> MSRSQLTILTNICLIEDLETQRVVMQYRAPENNRWSGYAFPGGHVENDEAFAESVIREIYEETGLTIQNPQLVGIKNWPL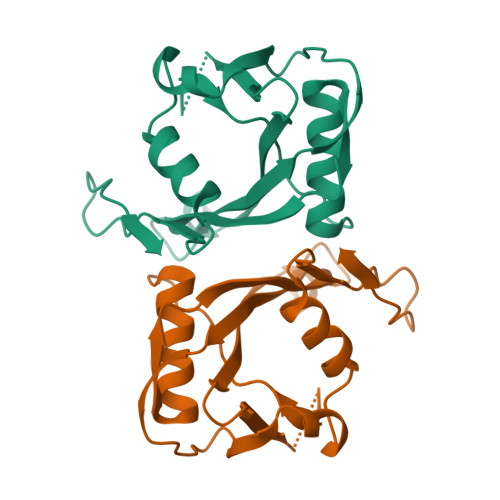DTGGRYIVICYKATEFSGTLQSSEEGEVSWVQKDQIPNLNLAYDMLPLMEMMEAPDKSEFFYPRRTEDDWEKKIF>MKLDIKKTFSNRSDRVKGIDFHPTEPWVLTTLYSGRVELWNYETQVEVRSIQVTETPVRAGKFIARKNWIIVGSDDFRIRVFNYNTGEKVVDFEAHPDYIRSIAVHPTKPYVLSGSDDLTVKLWNWENNWALEQTFEGHEHFVMCVAFNPKDPSTFASGCLDRTVKVWSLGQSTPNFTLTTGQERGVNYVDYYPLPDKPYMITASDDLTIKIWDYQTKSCVATLEGHMSNVSFAVFHPTLPIIISGSEDGTLKIWNSSTYKVEKTLNVGLERSWCIATHPTGRKNYIAS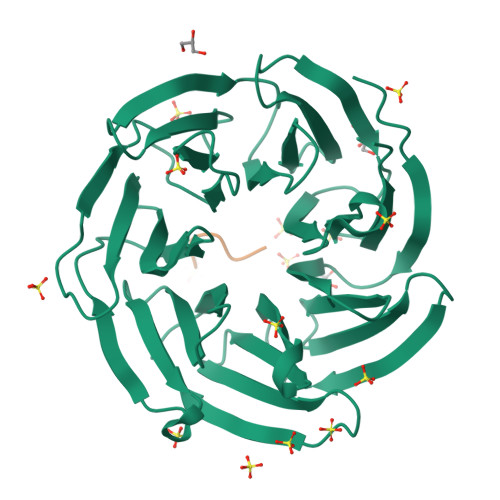GFDNGFTVLSLGNDE[24x];>LKIKKP[24x]>VSQNDIIKALASPLINDGMVVSDFADHVITRE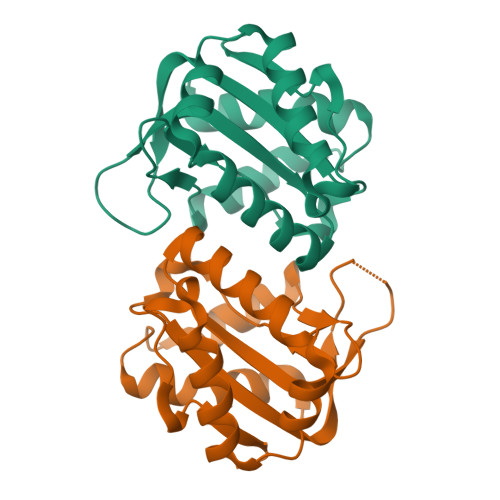QNAPTGLPVEPVGVAIPHTDSKYVRQNAISVGILAEPVNFEDAGGEPDPVPVRVVFMLALGNWFDITNVLWWIMDVIQDADFMQQLLVMNDDEIYQSIYTRISEAAGMAGIHFRRHYVRHLPLEHHHHHH[2x]5-methyluridine | 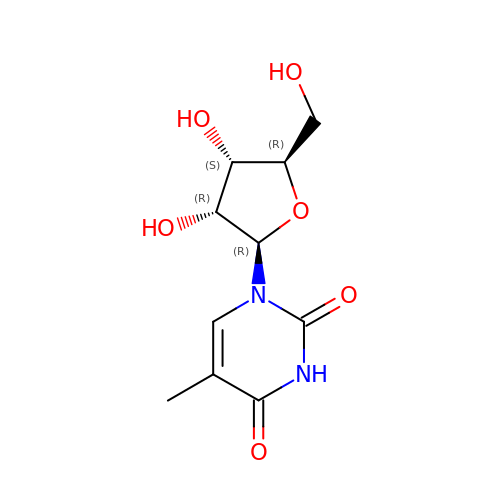C10 H14 N2 O6 | DWRXFEITVBNRMK-JXOAFFINSA-N> SNAMTEKKIDFKKEEKKFYAPKRKPERIFVPEMNFLMVDGKGDPDGEEYQKAVQSLYAIAYTIKMSKMGETRLDGYSDFVVPPLEGFWWSEGKFDLKDRDAWLWTSILRQPDFVTEEVLEWAKEVARKKKPDVDTSRVKLVRFEEGECVQMMHVGPFSEEVHTVAEMHQFMETEGLRNDTGAIRKHHEIYLSDPRKANPEKMKTILRLP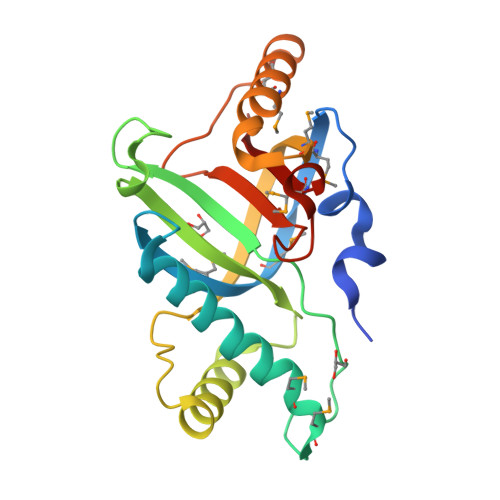VS>[2x]GPGSMVQFDVTIEIPKGQRNKYEVDHKTGRVRLDRYLYTPMAYPTDYGFIEDTLGEDGDPLDALVLLPEPLFPGVLVEARPVGMFRMVDEHGGDDKVLCVPVNDHR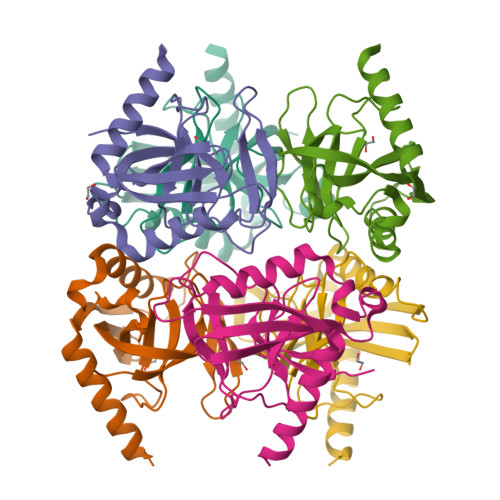WDHIHGIIDVPTFELDAIKHFFVHYKDLEPGKFVKAADWVGRDEAEAEVQRSVERFKAGGH>MNAKKRKGSAVERNIVSRLRDKGFAVVRAPASGSKRKDPIPDIIALKNGVIILIEMKSRKDGKIYVRREQAEGIIEFARKSGGSLFLGVKKPGVLKFIPFEKLRRTETGNYV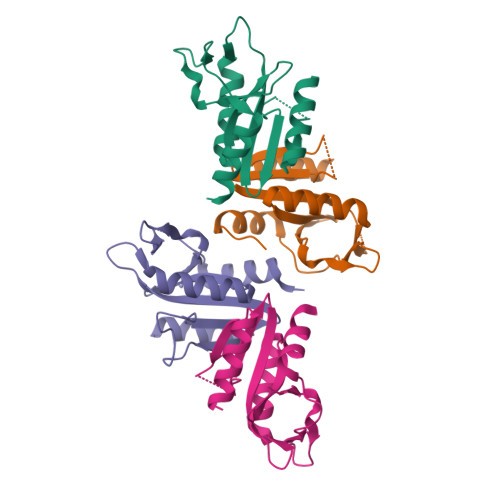ADSEIEGLDLEDLVRLVEAKISRTLDNFL[4x]>[2x]MEINVVRETMVRPAGATPQRVLWNSNVDLVIPRIHTASVYFYRPDPSGGEGYFEGGVLREALAKALVPFYPMAGRLKKDENGRFEINCNGEGVLLVEAAAANASVDEYARDFAPDVSFQRLIPSVDYTQDIGSFPLLVLQITRFKCGGASLGVGMEHHVADGMSGITFINTWAAMARGEDPKIVPYIDRTLLRANKPPIPKFPHVEYHPPPLLKHAAATNGHSNGKAKPQAGDDAPPRIAVGLFKFTKEQLQALKSQATDEETNTTYSSYEMLSGHIWRSMCLARGLDDDQETKLYIATDGRARVVPPLPKHYFGNVIFTCTPMALAGDLVSRPLYYAASVIHDAVSRMNDEYLRSALDYLELQPDLYKLVRGAHTFRSPNLGITSWSRLPVYDADFGWGRPVFMGPAVIAFEGLVYVLPSGTGDGSLSISLGLQPEHMPRFEQLIGQI

One interesting example is the hydroxycinnamoyl-CoA:shikimate hydroxycinnamoyltransferase (HCT), which belongs to the BAHD acyltransferase family involved in the biosynthesis of a diversity of ester- and amide-containing natural products. HCT produces p-coumaroylshikimate by transferring the p-coumaroyl group from the acyl donor p-coumaroyl-CoA to the acyl acceptor shikimate. It is an essential enzyme in the phenylpropanoid metabolism, conserved across all land plants. Interestingly, unlike many other essential metabolic enzymes, HCT exhibits relatively low affinity toward its native substrate shikimate and can utilize a variety of non-native substrates.

We crystallized the HCT ortholog from the lycophyte Selaginella moellendorffii and solved its apo structure at 2.9-Å resolution. The SmHCT crystal had a space group of P212121, and contained two molecules in the asymmetric unit. Several surface loops of the protein (residues 47-54, 216-237, and 259-262) have low electron density support and are omitted from the model. Similar to other HCT orthologs, the structure of SmHCT consists of two pseudo-symmetric domains: one comprised of residues 1-179 and 392-411, the other of 241-391 and 412-451, and a long intervening loop consisting of residues 180-240. The SmHCT active site is located at the interface between its two domains with a cavity volume of 1372.2±10.4 Å3. Inside the active site, the universally conserved catalytic His157 acts as a general base to deprotonate the 5-hydroxyl of shikimate, priming it for the subsequent nucleophilic attack on p-coumaroyl-CoA. Apart from His157, two other key residues involved in substrate binding and catalysis, Thr385 and Trp387, are also structurally conserved in SmHCT compared to other available HCT structures. However, there is a clear structural difference in the arginine handle, Arg372, which resides on one of the three short loops (L1) surrounding the entrance of the active site and coordinates the shikimate carboxylate with two salt bridges throughout the catalytic cycle. A lack of electron density for its side chain suggests that this residue is extremely flexible in SmHCT, occupying many different conformations in the apo state. This is in clear contrast to other crystallized HCT orthologs, which have defined density for the arginine handle.>MQSATQGKETATTTSSGTTYYVSSAHGDDANAGTSENAPWKSLTKVNDIASDLGPGDSVLLEYGSEFNDQYLHIKDTAGNADAPITISAYGDADEGKPVIASNGVKGSQWEQDYRANVGNHKNKGTVSTTLLLKDVSYITVSNLEITNDDADVYDPIDTWKWTDTPDSDGTKLDRSASRMDRTGVAGIAENGATMSNVTLDNLYIHDVDGNIYNKHMANGGIYFMAHYPMENTSAETDVWLREHVSRFDHVTIRNSTVKDVDRWGIAVGYTAYLNYIDANYGDGSIDDALIAKYGSTNVRIENNYVKGAGGDAITLMYCDRPVIEHNVGDSVSKHINTQDYTQPGSYGGRVAAGIWPWRCKDPVFQYNEMYNNLNAEHGNGDGQAWDADYGDGTLYQYNYSYGNSFASLMICNWYAVNTTFRYNISQNDRQGVFDLPSNGPGNHIYNNTVYVDADSQVLTKRSNSQSLFENNIFINATNTKKTETWNRGSQNGGQTYDNNMYVNYANKPTSDANAIEADDVSAVLAGAGSAPTSALKSGAEHARTGEKAAFDGYRPVAGSKAINAGKVVSDLNDYAV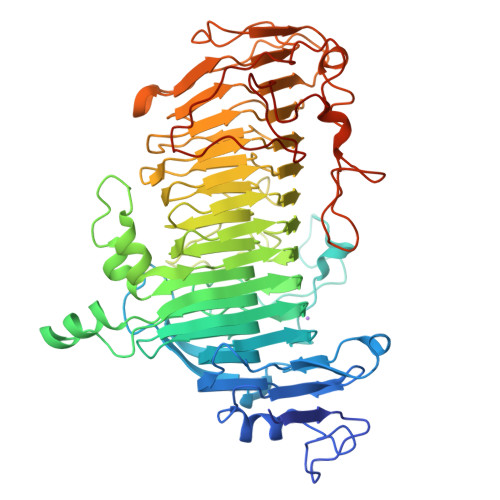ENDFLGNAVKGRPDLGAVEAALEHHHHHH[8x]Mitochondrial energy conversion requires an electron transport chain (ETC) that generates a proton motive force across the inner mitochondrial membrane to drive the essential adenosine triphosphate (ATP) formation by F1Fo-ATP synthase. The ETC consists of four multisubunit membrane complexes: complex I (CI; NADH:ubiquinone (UQ) oxidoreductase), complex II (CII; succinate:UQ oxidoreductase), complex III (CIII; cytochrome bc1) and complex IV (CIV; cytochrome c oxidase). We purified the intact respiratory supercomplex from mitochondria of the ciliate protist Tetrahymena thermophila and determined its structure by single-particle cryo-electron microscopy (cryo-EM). Here we show that a supercomplex containing all four respiratory chain components contributes to membrane curvature induction in ciliates.

CIII2 in our structure is tilted with respect to CI by 37°. This tilted arrangement offsets the transmembrane region, consistent with its curved membrane environment. We traced the membrane-accessible UQ tunnel, lined by UQCR10 and ciliate-specific subunit UQCRTT2, leading to the conserved COB haem bH, where the density for a bound (semi)-UQ was observed in the Qi site31. Furthermore, we observed map density features close to the two conserved haem bL groups, which probably correspond to ubiquinols bound at the Qo sites. The distances between the Qo site, haem bL and haem bH within each CIII monomer are consistent with those observed in mammalian CIII2, with the two haem bL in COB being bridged by a non-canonical UQ. We detected density for two copies of the flexible UQCRFS1 head domain, which contrasts with recent work that found only the head domain proximal to the CI quinone tunnel to display flexibility, whereas the distal domain at the CI interface was proposed to be non-functional in electron transport. Thus, our observation of the distal UQCRFS1 head domain flexibility, together with the haem bL-wedged UQ, suggests that functional symmetry is maintained in the ciliate CIII2 despite deviation from the structural symmetry.

>[2x]MFGRISQRISKLARLQRAFSTLQKQAQSNVVKSERLQFSKARLTDFGELPQGEIPTALQYDRPCRVETLANGVRLAVEPSSVSPLAAVSVVVRAGTRQETLETSGVAQFVQRLVLRGTSKRNREQIEKELALLGGNLKVQVGRETTTYTLSVLPENVEKAVDFLGDILQNSVFNKQQVEAEKEAVYNNALSAQNDQQGLLLENIHFTAYRDHYFGQPTHGIRENLHNITDEVVKNFVKTNYVGSNFVVAAAGNVNSQAFLQAAEKAFGTVAQKDATTFVPNTEKPYFTPSYMTIRDDEMHNLNVGVFFEAPSWTDPDFFTINFFQRILGEYQADKYTGQHLNTSDRQYSLIHKELGNLPDVTIHKTHYLPYSDTGLFGSYFYGNEIFGNQMLFLSQMILSEYASYINQAEIYRARAKYFNELLAEQNSADIASSIATQVTYLNRRVPRSEVAKRISSLDSGLINRAATRWFWDKELAIVTWGPSHGLIAGSHYNRSIKRSTLGWYGNTHYYIV;>MLSKITQNTLKSLSGQCKQAFSVRKAFYDFIYKDDKSAETYKVTTADPRTPVQGFRGQTAEDVAAKYEVTKLANGVTIITESQTFPSQVDMGILLDVGTRDETNETSGSLLSIKNTYLKTVLNTNETINYGVVQQSGGSFEMEYDQETAYFKANCLAHDATDVFSMVADCALEPRSTVAASVGVEKNQNTHKLESYLKTGELFNESVFKTAYGLKGLGLPLKGLRGNVKNLSSYTLQKFQLENITPNRIFVCAAGVESHQEFVDLVQTKLAQIPSAEGQKTHQREKSEYLGGEVRNLTEESNVTLALLFQSVPWSSADIVAFNVAAALLNNLRLKKNLLQKYAYFDQAEALNFHFTDSGLFGLRTSGSADRAKDILNHSIAELKAIASGVNADELLTAKAALKNSVLSALERQTDRLEETVKNVRTFNKIQHTDYVKQIDSVTADQVAKAVAKVLTSNPTFVAQGSQVNALPTYDAIRNLLK[2x];>MEWNKGTYMSTSIKKIVQYFSVMTVSFHDINSLFGFFTFLTIASQLVSGTMLAFSLVPEPMLIPMVREEEDVEDLYTDDFFWLHERGVDMLFIFSYFHLFRKIYLNNFEYEQEAAWKSGVFTFLLFQVVVFLGLVLCCTHLSDITLAIAANLYDTFFAGKGKFYWWIFTSKELNTDTIIRLAYLHYVLAFFLAYLGLIHGVDMHYDWKNESSMDGLETEMIWFDEALSNELGAMIEIILIVMIVCFFMYPEPEALSYEFFMWGDIGFINDVRFLSVAPHWYFRPFMAWLTVCPFHKIGLFGLIYYFFILFYQPVIHGTNEQNNYTKRNVAFVSFFINRSDIMTPKYHSVEDNLLHQITFWLFLCSALYVTSYLPYGRFYNRINGNYGTLWSFMYIFFYLGNSFLRRPLITELYLFNAFVKSKFLKK[2x];>MKSFVAAGIIGLSLANSQNKEVQNFIYRDDIGAFWGIKGYEELVTEVGTHKGHNYWPQFSFLGTYDSGSVRRGFQVFARNCGNCHGMIYKKYDYLLDKAYRQLELAQMVSDFTIHPAHQHFKQYYYQEWDERDRVICDHIYPPYFSQDQAKNANGGVWPTDFSKIKLRPGGINYIYNISTGYHFTPPFGMDVPKGKYFNPYFDHMIIGMPRQLVDGLVDYDDGTPASTPQMAYDVSNFINFMQRRVGYKRPDKMVRYYMVFTGGLLILPFKYFKTKAYYRNLLSLRWEMYAVRDGVYYNHFKYGGYNSRAYQFRGYFWA[2x];>MFSKTLAHVTRSCNKLNQVQAYNFGVLSEYNQRLSKKLHKGHLVEDKPTFFVTSSRPGNFGDHIDFKVNIDNWFDENRVHNEHETDIRRTQIYTLNAIYYGGLLSFARLYAMGVIGRLNGWKRYERDTYSEVDIGALPPGEVMQMVWNGTPIFIRRLTSNEVKEENELPSNTLLDKDKEVILSDAGNTKVIVVSAVCTHLGCIPIPYLGAYKGYVCICHGSVYDKFARVRQGPALLNLPAINNSIHDEGTLVCMEQLKFPHEPSQRFWA[2x];>MSNVSDAQIQEWIKRGEDPKEFLLKECAPQCTAWKEKLGRCEAKLKSLVNADPEMSCMYPLRDWVTCIEACVQPAITRNLFGSKYM[2x];>[2x]MVRLEKILWEQLVNVKAFSRQRVIGAPSKWYNENRTEWFKVAQHNAFNTGFSGVILRALEPLLAKFIYRWRLDIAHQRGLTLEDSLLFMDRELRRCYFFETVARQNLHPYTVLFMKKRRARYYKVERGLRGFYVPDWVRKEAEERQLSETVDNIFNWENFVYREYMSDMTPIGRWTSLSKITPLDMFQYYGLFRNEAWDRFFYNEAFYESYSEKEKQEANGNPFGKFNLQTADGRAQFEKEVNTFIERYPFAVTKPGQKFDFTRFYALEDLANKRDTSKYDPALLESVKNELKQSAALPADNGANKTKKSKPILPDWLQPKFGKAFQA;>[2x]MNVTGAGLTHVKDFHSDEMRVFRGGLRHIADKQGNLIYGSVNSSVRYYHDKMSYERGFIQHSRSPSNQFINFHFMLGGFRTYVLERFFKQVWYRRNIRTFWFPVLISYTSGCITMRMYDNNCYDYFYFSD;>MVYGKLIFNNIKEYTPSWIKTIPYSQVTKPILRKQPQIVGKINADPKVKKFWVFLRENVQYYPFLWQFFILGTSFVWFHVCYDPWLAIYQANNAHRSLETALTKEKAHKKKLAEQEESE[2x];>[2x]MYLPTFYKLFHETNAFRLKRYVGYGPLLLTWSIWTLYPALYNMIYSDFIPPERGVPKRIVDA;>[2x]MAPVFLKALRYVIYSYPLYVCYLIKQAQINAQGSEKEEEHH>[2x]SPNYDKWEMERTDITMKHKLGGGQYGEVYEGVWKKYSLTVAVKTLK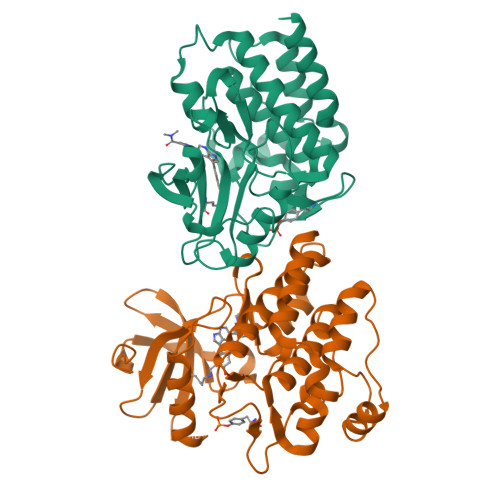EDTMEVEEFLKEAAVMKEIKHPNLVQLLGVCTREPPFYIITEFMTYGNLLDYLRECNRQEVNAVVLLYMATQISSAMEYLEKKNFIHRDLAARNCLVGENHLVKVADFGLSRLMTGDTYTAHAGAKFPIKWTAPESLAYNKFSIKSDVWAFGVLLWEIATYGMSPYPGIDLSQVYELLEKDYRMERPEGCPEKVYELMRACWQWNPSDRPSFAEIHQAFETMFQESSISD> MALERELLVATQAVRKASLLTKRIQSEVISHKDSTTIT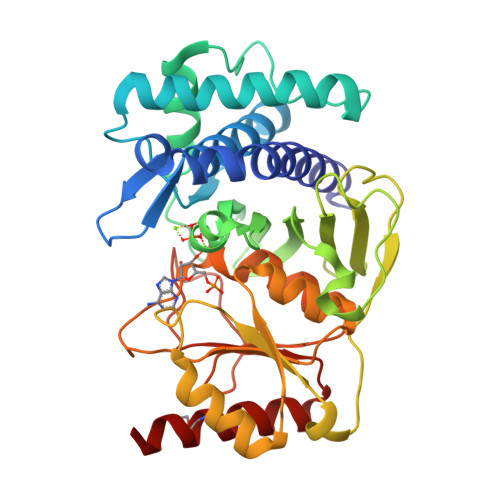KNDNSPVTTGDYAAQTIIINAIKSNFPDDKVVGEESSSGLSDAFVSGILNEIKANDEVYNKNYKKDDFLFTNDQFPLKSLEDVRQIIDFGNYEGGRKGRFWCLDPIDGTKGFLRGEQFAVCLALIVDGVVQLGCIGCPNLVLSSYGAQDLKGHESFGYIFRAVRGLGAFYSPSSDAESWTKIHVRHLKDTKDMITLEGVEKGHSSHDEQTAIKNKLNISKSLHLDSQAKYCLLALGLADVYLRLPIKLSYQEKIWDHAAGNVIVHEAGGIHTDAMEDVPLDFGNGRTLATKGVIASSGPRELHDLVVSTSCDVIQSRNA>MLQELRRELEELSVGSDGVLIWKIGSYGRRLQEAKAKPNLECFSPAFYTHKYGYKLQVSAFLNGNGSGEGTHLSLYIRVLPGAFDNLLEWPFARRVTFSLLDQSDPGLAKPQHVTETFHPDPNWKNFQKPGTWRGSLDESSLGFGYPKFISHQDIRKRNYVRDDAVFIRAAVELPRLEHHH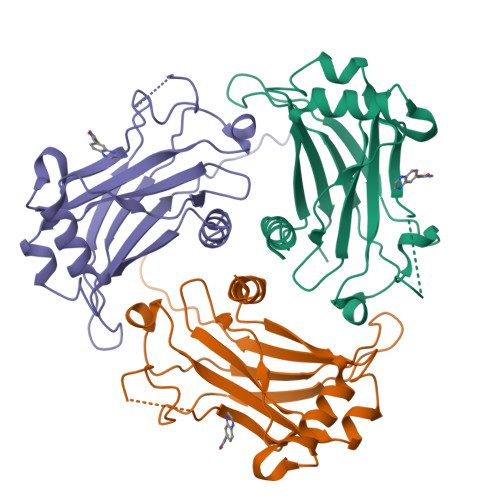H[3x]>[3x]MKNVYLPITVDHIARVEGKGGVEIVVGDDGVKE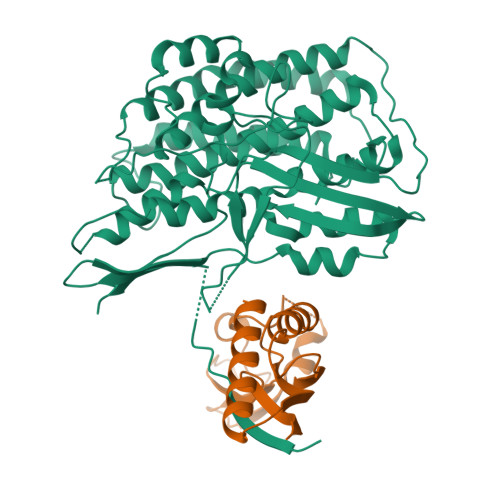VKLNIIEGPRFFEAITLGKKLDEALAIYPRICSFCSAAHKLTAVEAAEKAIGFTPREEIQALREVLYIGDMIESHALHLYLLVLPDYLGYSGPLHMIDEYKKEMSIALDLKNLGSWMMDELGSRAIHQENAVLGGFGKLPDKSVLENMKRRLKEALPKAEYTFELFTKLEQYEEVEGPITHIAVKPRNGVYGIYGDYLKASDGNEFPSEEYREHIKEFVVEHSFAKHSHYHGKPFMVGAISRLVNNADTLYGRAKELYESYKDLLRSTNPFANNLAQALELVYFTERAIDLIDEALAKWPIRPRDEVALKDGFGVSTTEAPRGVLVYALKVENGRVSYADIITPTAFNLAMMEQHVRMMAEKHYNDDPEKLKLLAEMVVRAYDPCISCSVHVARL;>MHEWALADAIVRTVLDYAQREGASRVKAVRVVLGELQDVAEDIVKFAMEQLFAGTIAEGAEIEFVEEEAVFKCRNCNYEWKLKEVKDKFDERIKEDIHFIPEVVHAFLACPKCGSHDFEVVKGRGVYVAGIKIEKEGGS[3x]>MASRGSHHHHHHGAGDRGPEFELGTRGSMNVYQLKEELIEYAKSIGVDKIGFTTADTFDSLKDRLILQESLGYLSGFEEPDIEKRVTPKLLLPKAKSIVAIALAYPSRMKDAPRSTRTERRGIFCRASWGKDYHDVLREKLDLLEDFLKSKHEDIRTKSMVDTGELSDRAVAERAGIGFSAKNCMITTPEYGSYVYLAEMITNIPFEPDVPIEDMCGSCTKCLDACPTGALVNPGQLNAQRCISFLTQTKGF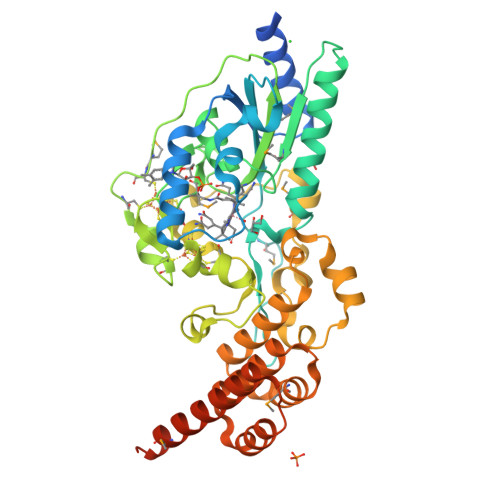LPDEFRTKIGNRLYGCDTCQTVCPLNKGKDFHLHPEMEPDPEIAKPLLKPLLAISNREFKEKFGHVSGSWRGKKPIQRNAILALAHFKDASALPELTELMHKDPRPVIRGTAAWAIGKIGDPAYAEELEKALEKEKDEEAKLEIEKGIELLKASGMTKQGLSGSLEVDLQGDHGLSAWSHPQFEK[2x]> MVEKGKMVKISYDGYVDGKLFDTTNEELAKKEGIYNPAMIYGPVAIFAGEGQVLPGLDEAILEMDVGEEREVVLPPEKAFGKRDPSKIKLIPLSEFTKRGIKPIKGLTITIDGIPGKIVSINSGRVLVDFNHELAGKEVKYRIKIEEVVD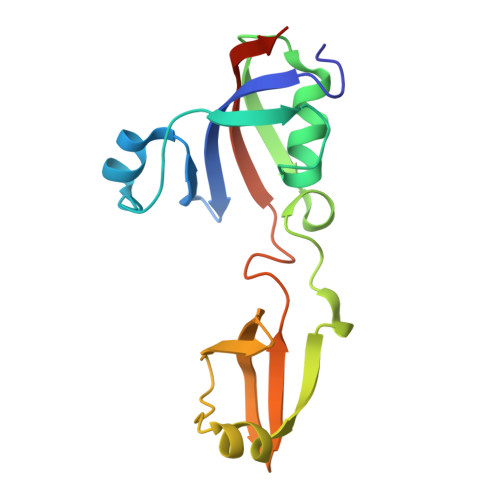LHHHHHH LOG produces active cytokinins via dephosphoribosylation, directly hydrolyzing the bond between N6-substituted bases and ribose 5′-monophosphates in cytokinin precursors such as iPRMP or trans-zeatin riboside 5′-monophosphate (tZRMP). Interestingly, C. glutamicum ATCC 13032 contains a gene product of Cg2612 that is annotated as a possible LDC (pfam03641) and a nucleotide-binding protein. Based on biochemical studies and structural comparison with other LOGs, we propose that Cg2612 functions as an LOG. On the other hand, EcCadA showed no phosphoribohydrolase activity with AMP as a substrate. These results confirm that Cg2612 belongs to the LOG family, and hereafter, we will represent Cg2612 as CgLOG.

To investigate the function of Cg2612, we determined its crystal structure at a 2.3 Å resolution. The asymmetric unit contained four molecules and seems to contain two distinct dimers. Interestingly, among four monomers in the asymmetric unit, two monomers contain a phosphate ion at each active site. We then performed small-angle X-ray scattering (SAXS) experiment to further confirm the dimeric conformation of Cg2612 in solution, and the result indicates that Cg2612 functions as a dimer as observed in other LOGs. The monomeric structure of Cg2612 shows an α/β fold belonging to a Rossmann fold. The central β-sheet which is formed by seven parallel β-strands is surrounded by eight α-helices. The dimerization interface is mainly composed of α5- and α6-helices, and the α4-helix partially aids in dimerization. Dimerization of two polypeptides constitutes a pocket which serves as the active site, and the conserved “PGGXGTXXE” motif was found in the surface of the pocket, which will be described in detail later. In our current structure, one phosphate and one glycerol molecule are bound at the AMP binding site and these molecules mimic the stabilization of the phosphate moiety and the ribose ring, respectively. Two proposed catalytic residues, Arg99 and Glu122, are located in the vicinity of the bond to be hydrolyzed; a covalent bond between adenine-N9 and ribose-C1.

>MTSLFDAPTLQRVTVFTGSALGSSSLYTQAAQTLAKTAVDRGIDLVYGGGKVGLMGIVADAFLESGGEAFGVITESLMKGELGHEKLTELEIVPDMHIRKRRMAELGDGFIAMPGGAGTLEELFEVWTWQQLGIHQKPVALYDVDGFWQPLLEMLEQMTQRGFIKRDFFECLIVESDPHALLKAMQTWTPPAPKWLEHHHHHH[4x]>[3x]AAPDEITTAWPVNVGPLNPHLYTPNQMFAQSMVYEPLVKYQADGSVIPWLAKSWTHSEDGKTWTFTLRDDVKFSNGEPFDAEAAAENFRAVLDNRQRHAWLELANQIVDVKALSKTELQITLKSAYYPFLQELALPRPFRFIAPSQFKNHETMNGIKAPIGTGPWILQESKLNQYDVFVRNENYWGEKPAIKKITFNVIPDPT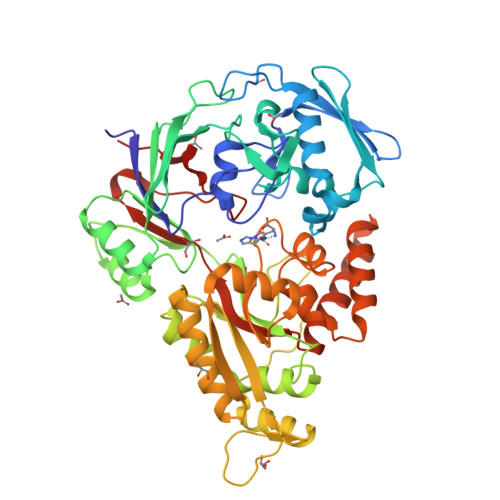TRAVAFETGDIDLLYGNEGLLPLDTFARFSQNPAYHTQLSQPIETVMLALNTAKAPTNELAVREALNYAVNKKSLIDNALYGTQQVADTLFAPSVPYANLGLKPSQYDPQKAKALLEKAGWTLPAGKDIREKNGQPLRIELSFIGTDALSKSMAEIIQADMRQIGADVSLIGEEESSIYARQRDGRFGMIFHRTWGAPYDPHAFLSSMRVPSHADFQAQQGLADKPLIDKEIGEVLATHDETQRQALYRDILTRLHDEAVYLPISYISMMVVSKPELGNIPYAPIATEIPFEQIKPVKP> MGSMVPSSPAVEKQVPVEPGPDPELRSWRHLVCYLCFYGFMAQIRPGESFITPYLLGPDKNFTREQVTNEITPVLSYSYLAVLVPVFLLTD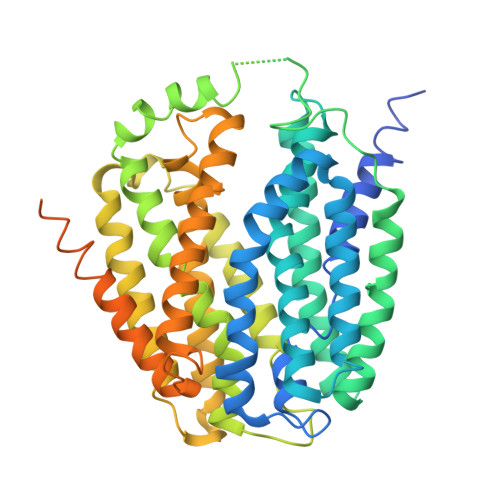YLRYTPVLLLQGLSFVSVWLLLLLGHSVAHMQLMELFYSVTMAARIAYSSYIFSLVRPARYQRVAGYSRAAVLLGVFTSSVLGQLLVTVGRVSFSTLNYISLAFLTFSVVLALFLKRPKRSLFFNRDDRGRCETSASELERMNPGPGGKLGHALRVACGDSVLARMLRELGDSLRRPQLRLWSLWWVFNSAGYYLVVYYVHILWNEVDPTTNSARVYNGAADAASTLLGAITSFAAGFVKIRWARWSKLLIAGVTATQAGLVFLLAHTRHPSSIWLCYAAFVLFRGSYQFLVPIATFQIASSLSKELCALVFGVNTFFATIVKTIITFIVSDVRGLGLPVRKQFQLYSVYFLILSIIYFLGAMLDGLRHCQRGHHPRQPPAQGLRSAAEEKAAQALSVQDKGLGGLQPAQSPPLSPEDKLGSENLYLEVLFQGPFQGGSGGSGHHHHHHHHHH[2-({4-[(2-amino-4-oxo-4,7-dihydro-3H-pyrrolo[2,3-d]pyrimidin-5-yl)methyl]benzene-1-carbonyl}amino)-4-methoxyphenyl]acetic acid | C23 H21 N5 O5 | 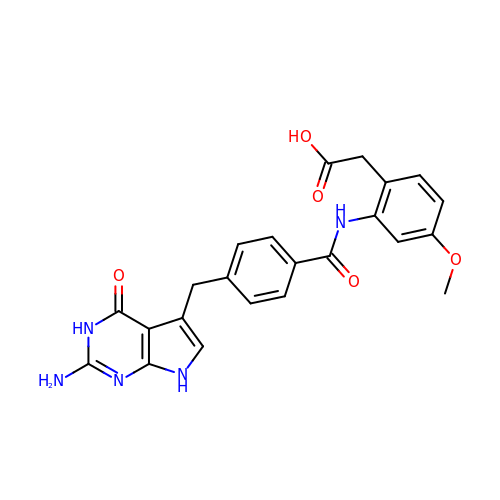UOZOJZZNBFZRTI-UHFFFAOYSA-N>MAHHHHHHMGDTFIRHIALLGFEKRFVPSQHYVYMFLVKWQDLSEKVVYRRFTEIYEFHKTLKEMFPIEAGAINPENRIIPHL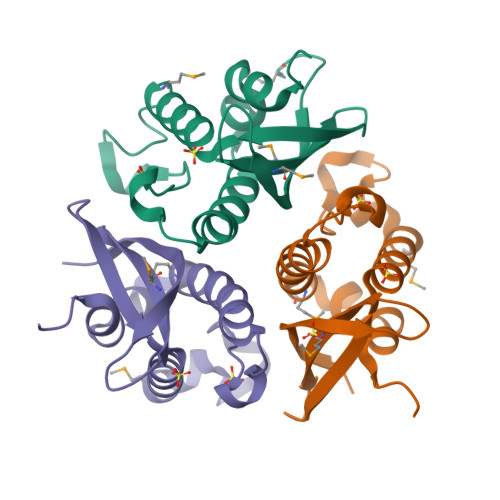PAPKWFDGQRAAENRQGTLTEYCSTLMSLPTKISRCPHLLDFFKVRPD[3x]>GSHMGIEYRSLHTSQLTLSEKEALYDLLIEGFEGDFSHDDFAHTLGGMHVMAFDQQKLVGHVAIIQRHMALDNTPISVGYVEAMVVEQSYRRQGIGRQLMLQTNKIIASCYQLGLLSASDDGQKLYHSVGWQIWKGKLFELKQGSYIRSIEEEGGVMGWKADGEVDFTASLYCDFRGGDQW[2x]

AAC(2′)-Ia is chromosomally restricted in Providencia stuartii, an opportunistic pathogen responsible for catheter-associated urinary tract infections with a high mortality rate. This enzyme is a part of a larger group of AAC(2′)-I isozymes, which includes five enzyme subtypes (AAC(2′)-Ia—AAC(2′)-Ie). Specifically, AAC(2′)-Ia utilizes cosubstrate, acetyl-CoA, to detoxify naturally occurring aminoglycosides such as kanamycin, tobramycin, sisomicin, and gentamicin, as well as semisynthetic aminoglycosides such as dibekacin, netilmicin, and plazomicin through the addition of an acetyl group at their 2′ positions.

Amikacin, a structural derivative of kanamycin, incorporates an (S)-HABA group at its N-1 position, but lacks an amine group at its N-2′ position, making it impervious to the effects of AAC(2′)-Ia (Ki = 87 ± 10 µM). The crystal structure of AAC(2′)-Ia in complex with acetyl-CoA and amikacin, a non-substrate aminoglycoside, is allowing us to capture the enzyme in a pre-catalysis state. In the pre-catalyzed state, the adenine rings of acetyl-CoA are sandwiched in between two flexible loops, with residue Arg89 on one side and Lys121 on the other; however, this portion does not form any inter- or intramolecular hydrogen bonds. Amikacin’s interactions are similar to those between the enzyme and its natural substrates. Although interactions are maintained, especially at the prime ring, the slight movement of residues around the active site in the amikacin-bound structure causes deviations in the positioning of the central and double-prime rings of the aminoglycoside. Additionally, the N-1 substitution does not form any hydrogen bond interactions with the enzyme, and instead, residues Glu148 and Glu149 shift to make it so the enzyme can accommodate the (S)-HABA group in a conformation away from the active site. The amikacin-bound structure shows that the enzyme is also capable of adapting the (S)-HABA moiety in a second conformation. This second conformation, as displayed by amikacin, exhibits that the N-1 tail can also sit parallel to the aminoglycoside plane. The adoption of this conformation is based on the movement of residue Glu149. Surprisingly, when comparing amikacin with plazomicin, different interactions are noted at the N-1 site. Both amikacin and plazomicin incorporate the (S)-HABA group at the N-1 position; however, while this moiety in amikacin does not form any specific interactions with the enzyme, the (S)-HABA tail of plazomicin forms hydrogen bonds with Glu149 and Asp176.> MKLLKDLLVDRKEFEDWKNNLTWARDGTLYLTTFPDISIGQPKYAKDINCNSKNLFHVKEFPLEFENKLDFELAQQNGLLNSQPVCYPRVCKPSPIDDWMAVLSNNGNVSVFKDNKMLTNLDSKGNLSSRTYHCFEWNPIESSIVVGNEDGELQFFSIRKNSENTPEFYFESSIRLSDAGSKDWVTHIVWYEDVLVAALSNNSVFSMTVSASSHQPVSRMIQNASRRKITDLKIVDYKVVLTCPGYVHKIDLKNYSISSLKTGSLENFHIIPLNHEKESTILLMSNKTSYKVLLEDELHVTADNIIAPYLEKKFKKWSTIWNEFNNYETTLVIHGISLSPDGYSIAIVYDMERVAFKYKIASEQSFNIMFAPLYHTWTISERAVGLAWYQTYQIYNQSLPKLPENFSMNKKLLNGNYPISLDFQSYLNALMKSEEMRIIMFLNMTIDKPSILSFLEALYEYAINKKSELTNSFDLACVLSIAAILKREAPIYNGTLLMKNSFLEETFNLESFTADPETVTSTTNNTWKRCGVTLLPILTTHVKICPVSK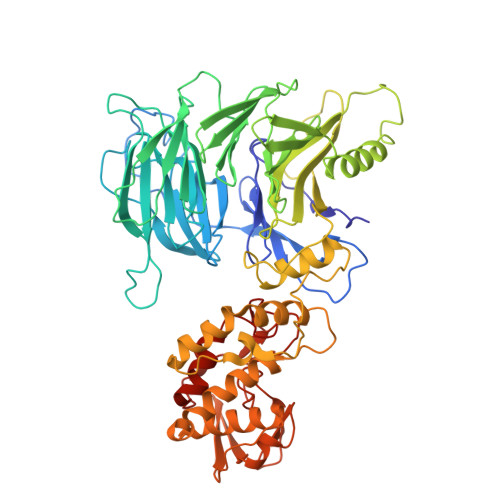QRVIDIKRDDLNDYGWFTRGLLERFNEISVYCGTTLEVM>GSHMSTITRPIIELSNTIDKIAEGNLEAEVPHQNRADEIGILAK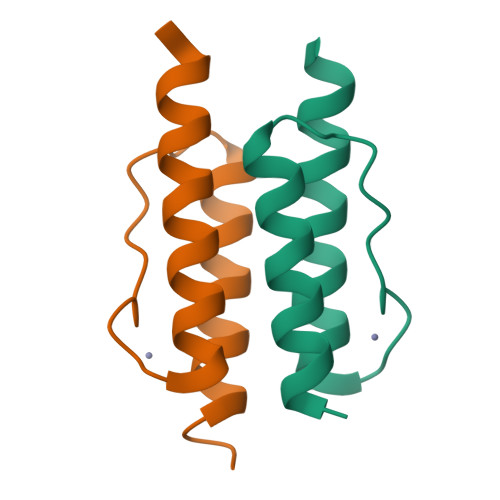SIERLRRSLKVAME[6x]>[4x]MASMTGGQQMGRGSMSRDPLPFFPPLYLGGPEITTENCEREPIHIPGSIQPHGALLTADGHSGEVLQMSLNAATFLGQEPTVLRGQTLAALLPEQWPALQAALPPGCPDALQYRATLDWPAAGHLSLTVHRVGELLILEFEPTEAWDSTGPHALRNAMFALESAPNLRALAEVAT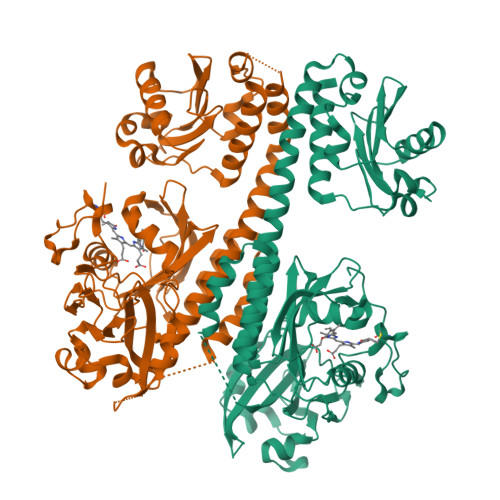QTVRELTGFDRVMLYKFAPDATGEVIAEARREGLHAFLGHRFPASDIPAQARALYTRHLLRLTADTRAAAVPLDPVLNPQTNAPTPLGGAVLRATSPMHMQYLRNMGVGSSLSVSVVVGGQLWGLIACHHQTPYVLPPDLRTTLEYLGRLLSLQVQVKEAADVAAFRQSLREHHARVALAAAHSLSPHDTLSDPALDLLGLMRAGGLILRFEGRWQTLGEVPPAPAVDALLAWLETQPGALVQTDALGQLWPAGADLAPSAAGLLAISVGEGWSECLVWLRPELRGGGSGYAEPWHPGEIEEAQDLRDTLTGALEHHHHHH>[2x]STLESKLNPSYISGFVDGEGSFMLTIIKDNKYKLGWRVVCRFVISLHKKDLSLLNKIKEFFDVGNVFLMTKDSAQYRVESLKGLDLIINHFDKYPLITKKQADYKLFKMAHNLIKNKSHLTKEGLLELVAIKAVINNGLNNDLSIAFPGINTILRPDTS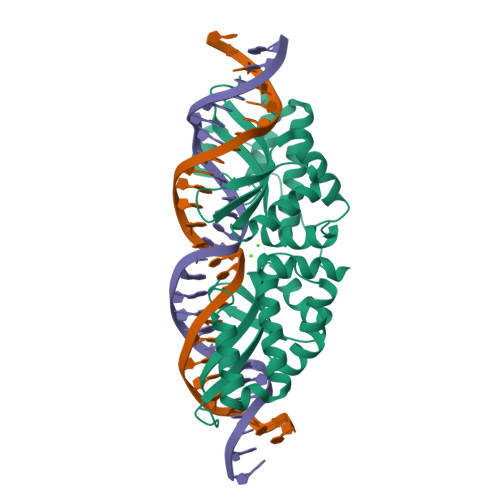LPQILNPFWLSGFVDAEGCFSVVVFKSKTSKLGEAVKLSFILTQSNRDEYLIKSLIEYLGCGNTSLDPRGTIDFKVTNFSSIKDIIVPFFIKYPLKGNKNLDFTDFCEVVRLMENKSHLTKEGLDQIKKIRNRMNTNRK6-amino-3-[(1S,3R)-4'-chloro-3-hydroxy-1',2'-dihydrospiro[cyclopentane-1,3'-pyrrolo[2,3-b]pyridin]-5'-yl]-2-fluoro-N,N-dimethylbenzamide 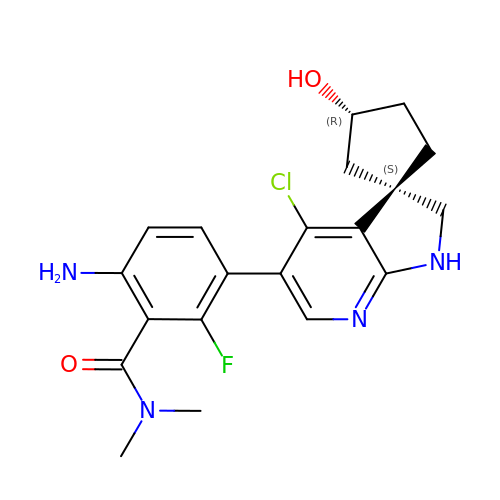| C20 H22 Cl F N4 O2 | PUEWEJKMMMXQTR-CFMSYZGJSA-N> MLNKKLDKKDKDAYPVESEIINLTINGVARGNHFNFVNGTLQTRNYGKVYVAGQGTSDSELVKKKGDIILTSLLGDGDHTLNVNKAESKELELYARVYNNTKRDITVDSVSLSPGLNATGREFSANKFVLYFKPTVLKKNRINTLVFGATFDEDIDDTNRHYLLSMRFSPGNDLFKVGEKLEHHHHHH

White spot syndrome virus (WSSV) is a rod-shaped enveloped virus with a large, double-stranded DNA genome, and belongs to the family Nimaviridae as the sole member of a novel genus Whispovirus56. For the interaction, VP24 has been recognized as a core protein to associate with other structural protein partners and form an envelope protein complex, serving as a hub protein to function in cell recognition, cell attaching and guidance of virus entry. Recently, VP24 has been demonstrated to be a chitin-binding protein involved in WSSV infection.

The transmembrane truncated VP24 (residues 28-208) was expressed and purified in E. coli BL21 (DE3) successfully. Lucky, after screening, with the addition of non-denaturing protein-solubilizing agent NDSB-201, soluble VP24 could reach a concentration of 3.5 mg/ml and yield crystals. Using SAD phasing, the crystal structure was determined to a resolution of 2.4 Å with a final Rwork of 0.17 and Rfree of 0.19 (refinement statistics see Table 1). The final monomer model of VP24 contains residues 40-208. The overall structure comprises nine β strands and one α helix, of which the nine antiparallel β-strands adopt a β–barrel fold to form the core of the protein, in which strand 9 is hydrogen-bonded to strand 1, and the short α helix on the turn between β3 and β4 is hanged out the β–barrel fold. The inner surface lining of the core is mainly contributed by the hydrophobic side chains from five Ile, seven Leu, five Phe, five Val, two Tyr and one Met residues; the hydrophobicity of the core is quite conserved among VP24, VP28 and VP26. In the crystal, VP24 forms a trimer by crystallographic three-fold symmetry axis. And the trimer interaction mainly contributed by β strands β1-β9-β6 and β7’. Furthermore, significantly different to those of VP26 and VP28, the N-terminus of VP24 forms a loop perpendicular to the barrel axis, which may pull the protein more closely attached to the viral envelope, compared to the protruding helix bundle parallel to the barrel axis of VP28. More interestingly, the electrostatic surface potential measurement of VP24 structure reveals an electronegative surface, owing to the presence of residues aspartate and glutamate residues at the top of β–barrel core (away from the viral envelope), and a highly electropositive surface at the bottom of the barrel core, distinct to those of VP28 and VP26.> MKPKVFITRAIPENGINMLEEEFEVEVWEEEREIPREKLLEKVKDVDALVTMLSERIDQEVFENAPRLRIVANYAVGYDNIDVEEATRRGIYVTNTPDVLTNATADHAFALLLATARHVVKGDKFVRSGEWKRKGIAWHPKWFLGYELYGKTIGIVGFGRIGQAIARRAKGFNMRILYYSRTRKSQAEKELGAEYRPLEEVLKESDFVILAVPLTKETMYMINEERLKLMKPTAILVNIARGKVVDTKALIKALKEGWIAGAGLDVFEEEPYYNEELFSLDNVVLTPHIGSATF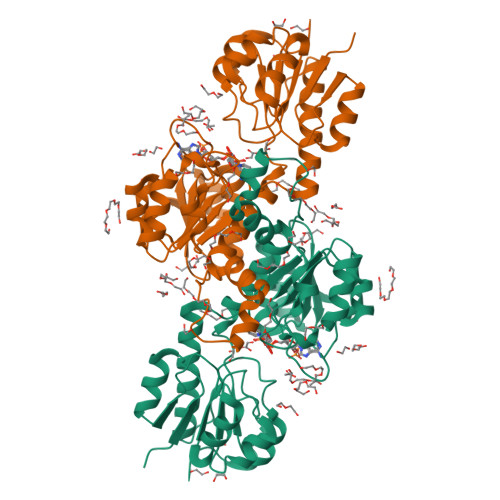EAREAMAELVARNLIAFKRGEIPPTLVNKEVIKIRKPGFNEQ>MADDQGCIEEQGVEDSANEDSVDAKPDRSSFVPSLFSKKKKNVTMRSIKTTRDRVPTYQYNMNFEKLGKCIIINNKNFDKVTGMGVRNGTDKDAEALFKCFRSLGFDVIVYNDCSCAKMQDLLKKASEEDHTNAACFACILLSHGEENVIYGKDGVTPIKDLTAHFRGDRCKTLLEKPKLFFIQACRGTELDDGIQAD[2x];>SGPINDTDANPRYKIPVEADFLFAYSTVPGYVSMRSPGRGSWFVQALCSILEEHGKDLEIMQILT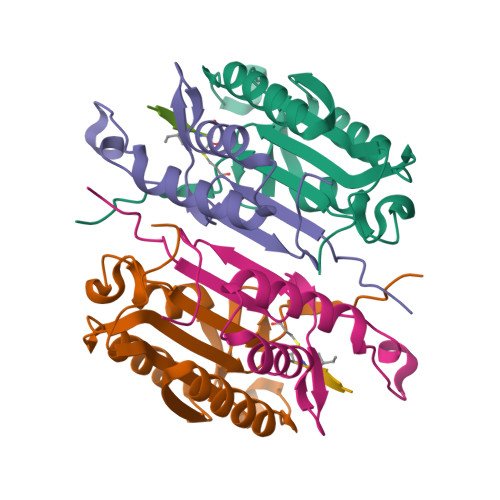RVNDRVARHFESCSDDPHFHEKKQIPCVVSMLTKELYFSQLEHHHHHH[2x];>[2x]XVEID>[2x]SFKRDGDDLVYEAEIDLLTAIAGGEFALEHVSGDWLKVGIVPGEVI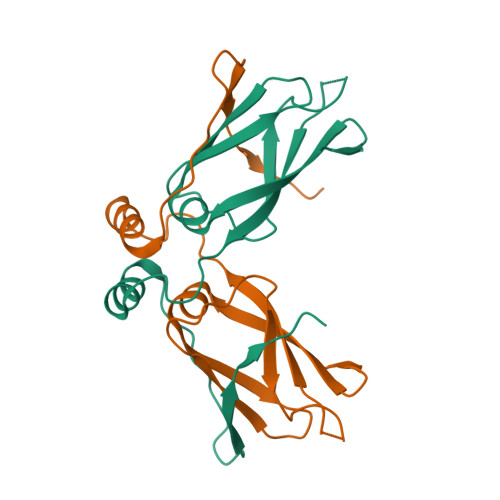APGMRKVIEGKGMPIPKYGGYGNLIIKFTIKFPENHFTSEENLKKLEEILPPRIVPAIPKKATVDECVLADFDPA>MSKIERISAFLNDKEVDMTFITNPTTLNYLTGLAIDPHERIAGLMIFRDSTPMLFTPALEVEKAKEHTSGLDIFGYEDSQNPWEVVKNHVKSDVKSIAVEFSDIPLAKTEGLKAQFGDINFVNLTPLIERMRLIKSADEIEKMKVAGDFADKCFEIGFATAAERNGVTESDIVAKIEYEMKRMGVPQMSFDTLVLSGARAANPHGAPENVEIQENKLLLFDLGVMSGGYASDATRTIAIGQPNDFDAEIHKIVKEAQQAAMDFIKPGVTAHEVDAVARDLITKAGYGEYFNHRLGHGIGMDVHEYPSIVAGNDLVIQEGMCFSNEPGIYIPGKVGVRI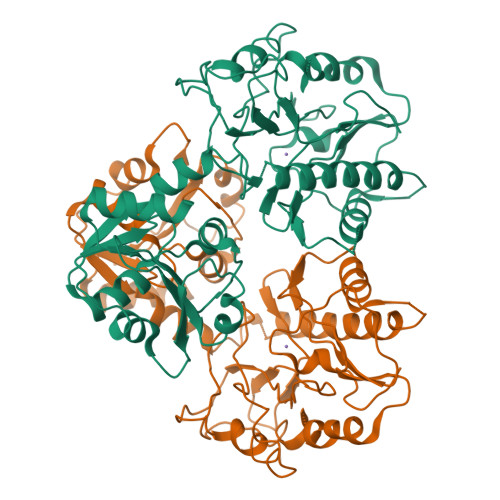EDCLYVTENGCESFTHTDHDLLIF[3x]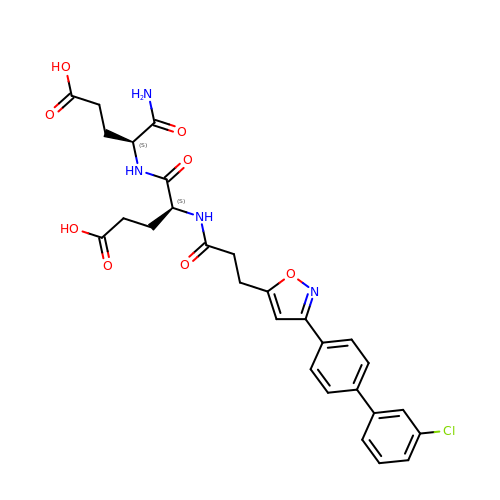N-{3-[3-(3'-chlorobiphenyl-4-yl)isoxazol-5-yl]propanoyl}-L-alpha-glutamyl-L-alpha-glutamyl-amide | C28 H29 Cl N4 O8 | KOVQMCGGWATESY-VXKWHMMOSA-N> MAKKKIKRRGKMPPNIFDTGGQSWGQQSSGQFSNAFKGENLGNSIGSIGGAVGGIAQAGISNAQIADTSGIEAQNKAQKNMVVGASSNDDLMSEWGSWNKVKDDYSWKDVRGGSTGQRVTNTIGAAGQGAAAGASVGGPIGAIVGGVVGLGSAIGGWLGGNRKAKRKAKKLNKEAKEANERALTSFETRADNIDTQNDF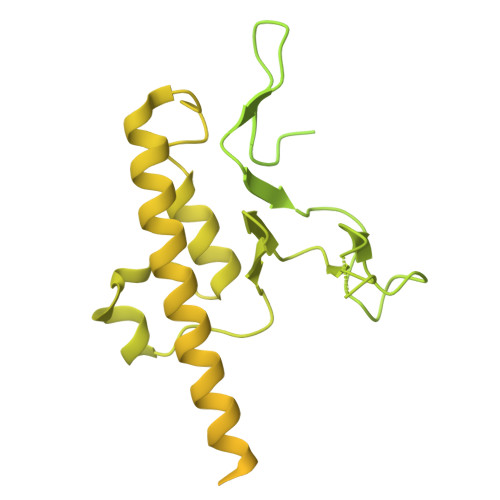NMLANFSAYGGPLEFGSGAIGYEFDNRYLNNQEMSAVAKQRLTSLPNSFQALPEMNTYNAFAEGGGLSREKNYGSKKKPYPSVPSGDFAGPHRSYPIPTKADARDALRLAGLHGNESVRRKVLAKYPSLKAFGGSLFDSVVGNNFNQSFTQGIQGMFQQEPEQTVQAANIAKDGGDIKIKEKNKGKFTAYCGGKVTEACIRKGKNSSNPTTRKRATFAQNARNWNAFGGWLNTQGGDFTNGVTFINEGGSHEENPYQGIQIGVDPEGAPNLVEQGEVVYDDYVFSDRMEIPDDIRKEYKLRGKTFAKAAKSAQRESEERPNDPLSTKGLQAAMERIATAQEEARQRKEAHREGNEYPSMFAYGGDTNPYGLALEDPMSVEELEALMVQSGETGEIAPEGNNGNRQTWTRYAPIIGSGLASLSDLFSKPDYDSADLISGVDLGAEAVGYAPIGNYLSYRPLDRDFYINKMNQQAAATRRGLMNTSGGNRLNAQAGILAADYNYGQNMGNLARQAEEYNQQLRERVEAFNRGTNMFNTETGLKASMFNAESRNAAKRARLGQATTVAQLRQGIKDQDAARRSANITNFLQGLGDMGWENEQANWLDTLAKSGVLKMNTKGEYTGGTKKAKGGKVRTKKKKGLTYG4-(2-anilinopyridin-3-yl)-N-(3,4,5-trimethoxyphenyl)-1,3,5-triazin-2-amine 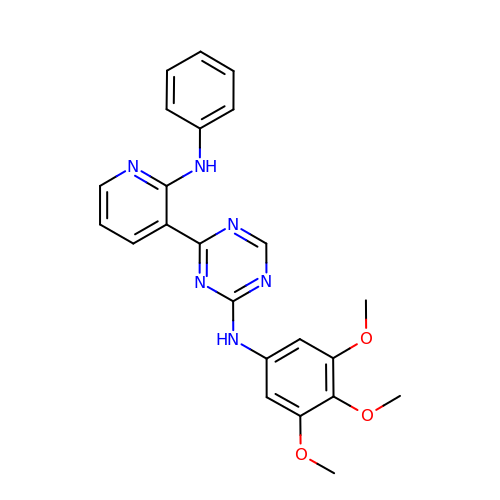| C23 H22 N6 O3 | YRSYWYSGZPRSOP-UHFFFAOYSA-N> MGSHHHHHHSQDPMMSRLKTAVYDYLNDVDI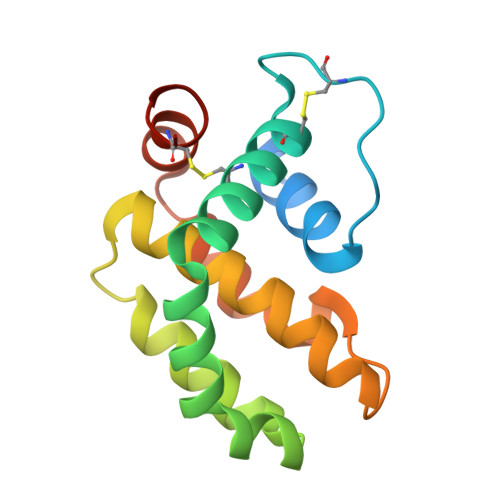TECTEMDLLCQLSNCCDFINETYAKNYDTLYDIMERDILSYNIVNIKNTLTFALRDASPSVKLATLTLLASVIKKLNKIQHTDAAMFSEVIDGIVAEEQQVIGFIQKKCKYNTT>MVQKWMQRMIIVDNNKLNVRALPSFIDYFNGIYGFATGIKDIMGMIFKTDTGGSNLTLDEILKNQNLLNDISGKLDGINGDLGDLIAQGNLNSELAKELLKISNEQNQMLNHVNAQLNAINSTLNIYLPKITSMLNEVMKQNHVLSLQIEFLSKQLQEISDKLDIINLNVLINSTLTEITPAYQRIKYVNEKFDELTSTVEKNPKSYQDNVTKEVIENLNELTELAKSVTKNDMDSFEFYLQTFHDVMTGNNLFGRSALKTASELITKENVTTRGSEIGKVYNFLIVLTSLQAKAFLTLTACRKLLGLTDIDYTQIMNHHIDGQKREFRINILPTLSNNFSNPSYSKNRGSDIDDPIVVLEAAPGYALIGFEILNDPLPILKGYQARLKPNYQVDRESMSETIYGDIHKLFCPKQLEQKYYIKDIEFPEGYVITKIVFEKRLNQLGYEVTANFYDPSTGSIDLNKVKVESWKEKSCEEDSCEDEYSIIKAETDGIYMPLGVVSETFLTPIYGFGLTVDEKNQKITLTGKSYLRESLLETDLLNNETYLIASPDGYISSIVENWNITSDNTGSWR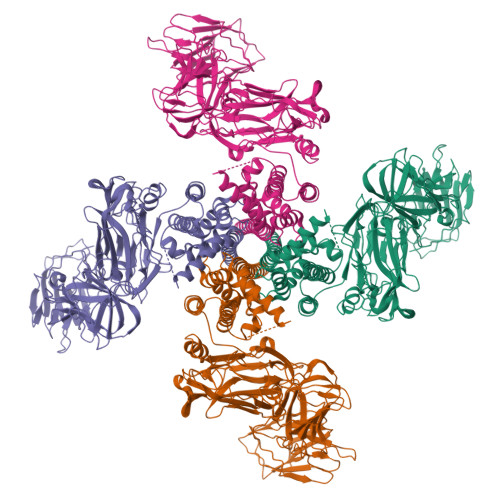ANNNNAFVDKADTIKGSSSLYTHKDGEFSQFIGNKLKPKTNYVIQYVIKGRPAIYLKNNKDTLFEDTKNNFSDFQTVTKKFNSGVNPSEIYFLFKNQSEYEAWGNNFIILEIKSLEFLPQMLKPEDWIPSGNVQMKDGGRLEILGDGYFKQFIKLENDSTYHLRLSVKGTGRVSIIDESKYLLFVNVKDEDLTRVIKNTSSKGECFIALEGTYVENSSTIFSNVSIVKE[4x]A glucosylglycerate hydrolase (GgH) identified in M. hassiacum and found to be highly conserved among rapidly growing mycobacteria is likely to be responsible for the rapid mobilization of GG accumulated during nitrogen starvation by hydrolysing it to glucose and glycerate. The MhGgH monomer displays an (α/α)6-barrel domain typical of glycoside hydrolase family 63 (GH63), to which MhGgH belongs. While the active site of GH63 members acting on larger substrates is located in an open, solvent-accessible cleft, those of MhGgH and of MgH from T. thermophilus are covered by a cap domain (subdivided into A′- and B′-regions) with constrained access through a narrow negatively charged tunnel. The crystallographic structure of MhGgH revealed a homotetrameric architecture, which is compatible with the oligomeric organization of the enzyme in solution as assessed by SAXS.

To avoid substrate hydrolysis during crystallization or soaking, three catalytically inactive variants of MhGgH were produced. Two putative catalytic residues (Asp182 and Glu419) and one substrate-interacting residue (Asp43) were identified and replaced by alanine to produce the D43A, D182A and E419A variants. The thermal stability of the D182A and E419A variants was comparable to that of wild-type MhGgH, while that of the D43A variant was slightly lowered (3°C) [Fig. 2(d)]. During hydrolysis, the negatively charged Glu419 is likely to activate the water molecule that performs a nucleophilic attack on the anomeric C atom, while Asp182 donates a proton to the leaving glycerate.

>GAMPHDPSFTPTQLAARAAYLLRGNDLGTMTTAAPLLYPHMWSWDAAFVAIGLAPLSVERAVVELDTLLSAQWRNGMIPHIVFANGVDGYFPGPARWATATLADNAPRNRLTSGITQPPVHAIAVQRILEHARTRGRSTRAVAEAFLDRRWGDLMRWHRWLAECRDRNERGRITLYHGWESGMDNSPRWDSAYANVVPGKLPEYQRADNVIITDPSQRPSDGEYDRYLWLLEEMKAVRYDDERLPSVMSFQVEDVFFSAIFSVACQVLAEIGEDYKRPHADVKDLYLWAERFRAGVVETTDQRTGAARDFDVLAEKWLVTETAAQFAPLLCGGLPHDRERALLKLLEGPRFCGHPDLKYGLIPSTSPVSRDFRPREYWRGPVWPVLTWLFSWCFARRGWAERARLLRQEGLRQASDGSFAAYYEPFTGEPLGSMQQSWTAAAVLDWLG[2x]N,N-dimethyl-2-(methylsulfanyl)pyridine-3-carboxamide | C9 H12 N2 O S | 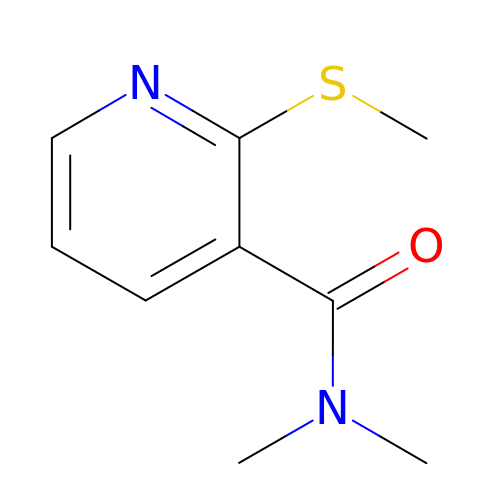KORZBTDVYBSAMM-UHFFFAOYSA-N> MDGSGEQPRGGGPTSSEQIMKTGALLLQGFIQDRAGRMGGEAPELALDPVPQDASTKKLSECLKRI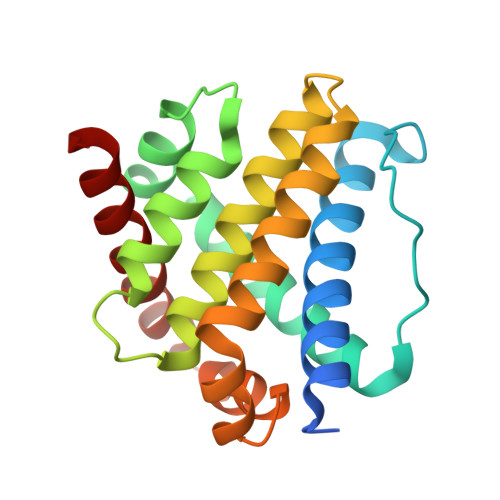GDELDSNMELQRMIAAVDTDSPREVFFRVAADMFSDGNFNWGRVVALFYFASKLVLKALCTKVPELIRTIMGATLDFLRERLLGWIQDQGGWDGLLSYFGTPTWQTVTIFVAGVLTASLTIWKKMG> MEQANPLRPDGESKGGVLAHLERLETQVSRSRKQSEELQSVQAQEGALGTKIHKLRRLRDELRAVVRHRRASVKACIANVEPNQTVEINEQEALEEKLENVKAILQAYHFTGLSGKLTSRGVCVCISTAFEGNLLDSYFVDLVIQKPLRIHHHSVPVFIPLEEIAAKYLQTNIQHFLFSLCEYLNAYSGRKYQADRLQSDFAALLTGPLQRNPLCNLLSFTYKLDPGGQSFPFCARLLYKDLTATLPTDVTVTCQGVEVLSTSWEEQRASHETLFC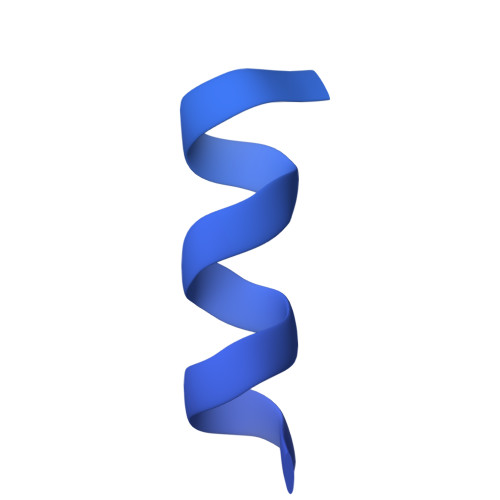TKPLHQVFASFTRKGEKLDMSLVS> VEPSGHAADRIARLPGQPAVDFDMYSGYITVDEGAGRSLFYLLQEAPEDAQPAPLVLWLNGGPGCSSVAYGASEELGAFRVKPRGAGLVLNEYRWNKVANVLFLDSPAGVGFSYTNTSSDIYTSGDNRTAHDSYAFLAKWFERF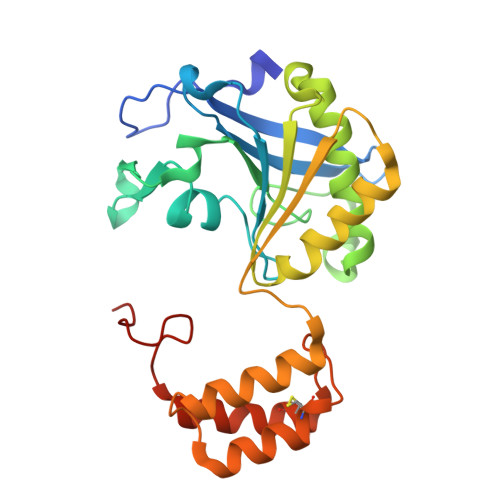PHYKYRDFYIAGESYAGHYVPELSQLVHRSKNPVINLKGFMVGNGLIDDYHDYVGTFEFWWNHGIVSDDTYRRLKEACLHDSFIHPSPACDAATDVATAEQGNIDMYSLYTPVCNITSS>[4x]MIVILDNGGQYVHRIHRSLKYIGVSSKIVPNTTPLEEIESNKEVKGIILSGGPDIEKA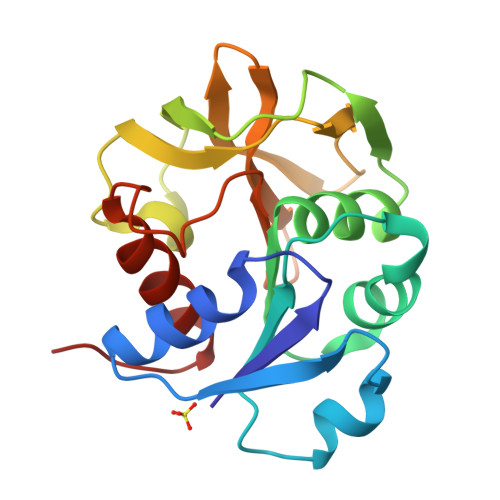KNCIDIALNAKLPILGICLGHQLIALAYGGEVGRAEAEEYALTKVYVDKENDLFKNVPREFNAWASHKDEVKKVPEGFEILAHSDICQVEAMLHKTKPIFGVQFHPEVAHTEYGNEILKNFCKVCGYKFE> RTVFSSLTVNGVDLGQGVAVRVPSSNAPVTDIESDDIICNTGFIQPVSKTVAAVPAGGTVIAHFH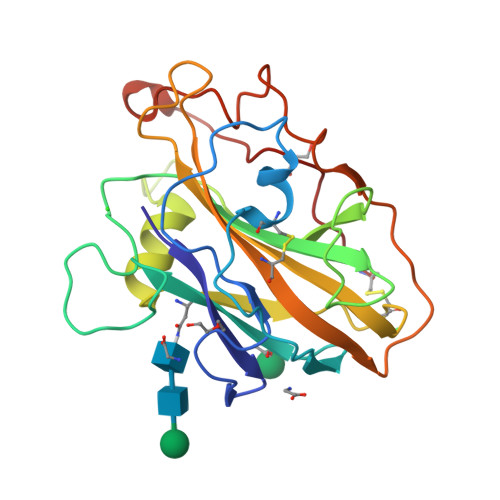HTSAGYVGPDPSDPLDPTNKGPVLAYLAKVPDATQSDVTGLKWFKIWQDGYTPATRQWGSDKLFINGGNATFTIPSCLQAGQYLLRVESISLLNAEQYPGAQFFLSCGQINITGGNKVQPVGVDFPGAYTSTDPGIVTDIYEVGTYTPPGPAVFSC oxidoreductase family that is found in all three domains of life. trans-to-cis isomerization of the Ile75-Pro76 peptide bond. specific conformation and local environment of its active-site cysteine pair.

possible mechanism through the replacement of all prolines by alanine. rearrangements in the segments 39–41 and 92–95. Trx0P at 25 °C and pH 7.0. Trx WT, and that Trx0P is more oxidizing than Trx1P. redox potential of Trx0P relative to Trx WT and Trx1P. 75–76 bond thus made Trx0P a significantly worse substrate of TrxR. as DTT reduced Trx0P even faster than Trx WT. completely abolished the function of the protein as electron transfer catalyst. independent evidence for a Trx0P-like tertiary structure of Itrans.

>[3x]SDKIIHLTDDSFDTDVLKADGAILVDFWAEWCGACKMIAAILDEIADEYQGKLTVAKLNIDQNAGTAAKYGIRGIATLLLFKNGEVAATKVGALSKGQLKEFLDANLA>VRRDRAPPERGGAGTSQDGTSKNWFKITIPYGRKYDKAWLLSMIQSKCSVPFTPIEFHYENTRAQFFVEDASTASALKAVNYKILDRENRRISIIINSSAPPHTILNELKPEQVEQLKLIMSKRYDGSQQALDLKGLRSDPDLVAQNIDVVLNRRSSMAATLRIIEENIPELLSLNLSNNRLYRLDDMSSIVQKAPNLKILNLSGNELKSERELDKIKGLKLEELWLDGNSLCDTFRDQSTYISAIRERFPKLLRLDGHELPPPIAFDVEAPTTL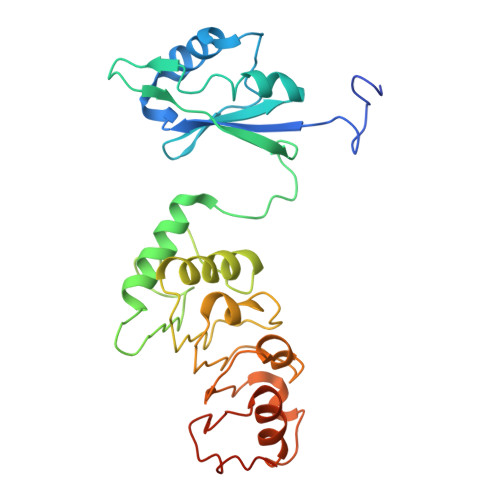PP[4x]>[4x]S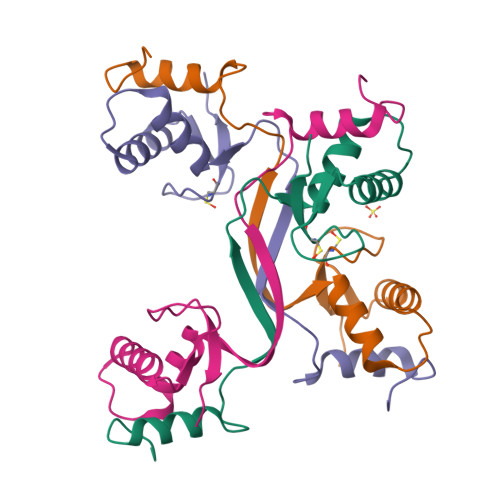SGLSVHTDMASVTKAMAAPESGLEVRDRMWLKITIPNAFLGSDVVDWLYHHVEGFPERREARKYASGLLKAGLIRHTVNKITFSEQCYYVFGDLSG>[10x]MHHHHHHMQGSIPMAGPPDSDLDDVARI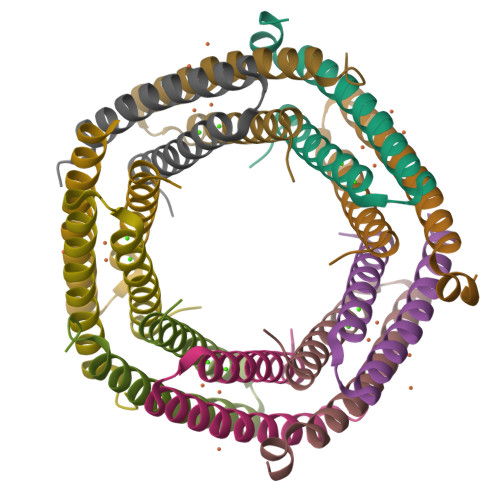RLVLARELETINEYEAYARASSNPEVRAFFQHLAAEEKEHVSEAVHMLRMLDSGQNDHFAKPFVPGHFQAAEAPAPATV>GAMASGGDPKWQKDAADQNFDYMFKLLIIGNSSVGKTSFLFRYADDSFTSAFVSTVGIDFKVKTVFRHDKRVKLQIWDTAGLERYRTITTAYYRGAMGFILMYDVTNEDSFNSVQDWVTQIKTYSWDNAQVILVGNKCDMEDQRVISFERGRQLADQLGVEFF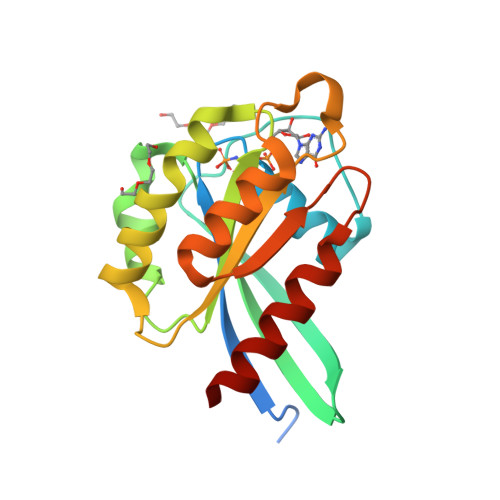ETSAKENVNVKAVFERLVDIICDKMSE[2x]>GSMTNIPFIYQYEEKENERAAAGYGTFGYLITRIEETLYDQYGVFYELYASDDPNTEYWELLVEDVRSGSLEPEHVAYIFEKLEKKTFAYDEDEKEPDYTVHKSIRNSVYAYPEKGVAFARIPYFQDGSIMSFDCLFAVNDEKMRAFLEGVRPRLWEKSKRKVTVFTDGDGGTSREQEAIVREVQRSQVIMNPLLKKEIYRSIDQFFHSDKSFYQTYDIPYKRGILLYGPPGNGKTTLVKSIAGSIDAPVAYWQITEFTSSETIEEVFQAARRLAPAVLVIEDIDSMPEDVRSFFLNTLDGATS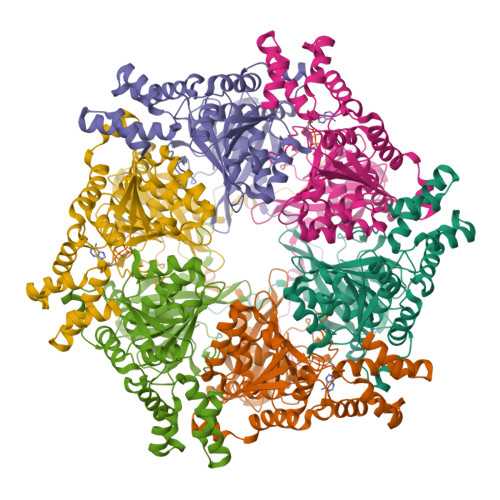KEGLFLIGTTNYPEEIDPGLMNRAGRFDRAYEIGLPDEELRLEYMKMRGFGIFLSEGEIKNAAKLTEGFSFAQLGELYVSSALQWHQEGNHHIETMVKDMTGEQRKSQRGSWMERNKVGFH[2x]>AQKSVKISDDISITQLSDKVYTYVSLAEIEGWGMVPSNGMIVINNHQAALLDTPINDAQTEMLVNWVTDSLHAKVTTFIPNHWHGDCIGGLGYLQRKGVQSYANQMTIDLAKEKGLPVPEHGFTDSLTVSLDGMPLQCYYLGGGHATDNIVVWLPTENILFGGCMLKDNQTTSIGNISDADVTAWPKTLDKVKAKFPSAR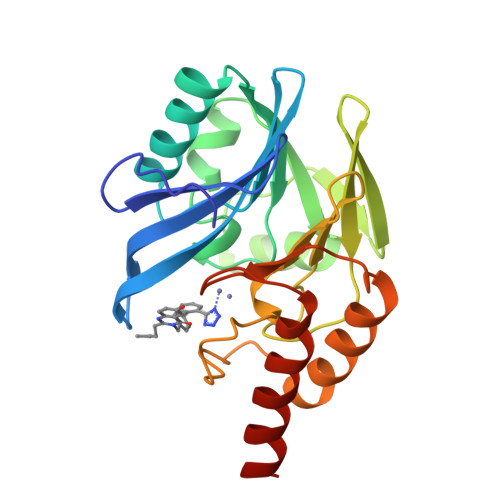YVVPGHGNYGGTELIEHTKQIVNQYIESTSKP[2x]Protoglobin (Pgb) is a recently discovered haem-protein with distinct structural and functional features that make it unique within the globin superfamily. The MaPgb* structure can be considered as an expanded version of the 3/3 helical sandwich typical of “classical” globins (i.e. Mb), with an additional N-terminal extension, built by a 20-residue loop, followed by the Z-helix, which precedes the globin-fold conserved A-helix. Residues belonging to the Z-helix contribute to formation of the Pgb homodimer, which is centered on the intermolecular four-helix bundle built by the G- and H-helices of the two subunits. Thus, in Pgb the access of diatomic ligands, such as O2, CO, and NO, to the haem is granted by two orthogonal apolar tunnels that reach the haem distal region from entry sites at the B/G and B/E helix interfaces.

High-resolution data (1.60 Å) on the MaPgb*(III)-cyanide crystals were collected at the ESRF synchrotron facility (ESRF, Grenoble, France), and the structure was refined to a final R-factor and R-free of 17.5% and 23.8%, respectively. In the MaPgb*(III)-cyanide complex the cyanide molecule is bound to the sixth coordination site of the haem-Fe(III) atom, with a coordination bond of 2.16 Å and a Fe-C-N angle of 171° for chain A, and of 2.14 Å and 169° for chain B. Two H-bonds stabilize the haem-Fe(III)-bound cyanide molecule. On one hand, the cyanide N atom is linked to Tyr(61)B10 OH group (2.84 Å and 2.71 Å, for chain A and B, respectively), on the other, it is hydrogen bonded to Trp(60)B9 Nε2 atom (2.98 Å or 2.99 Å). The presence of the haem-Fe(III)-bound cyanide molecule induces a rotation of the Phe(93)E11 side chain around the Cβ-Cγ bond of about 120° relative to the ligand-free MaPgb*(III). The rotation of the Phe(93)E11 side chain allows the rotation of the Trp(60)B9 side chain of ∼90° towards the center of the haem distal site. As a consequence, in the MaPgb*(III)-cyanide complex: (i) tunnel 1 is hindered by the Trp(60)B9 side chain, and (ii) the Trp(60)B9 Nε1 atom is at H-bond distance to the haem-Fe(III)-bound cyanide ligand. Interestingly, the 149–154 region, which faces Trp(60)B9 side chain on one side and the second subunit of the dimer on the other, is significantly divergent in its Cα-backbone relative to the ligand-free MaPgb*(III) and MaPgb*(II)-O2 structures (maximum displacement at Ala(151)G13 of 1.75 Å and 1.64 Å, respectively), and shows signs of structural heterogeneity, with Ile(149)G11 and Thr(152)G14 adopting two alternate conformations. Thus, ligand binding, and the consequent relocation of the Trp(60)B9 side chain within the haem distal cavity, appears to release structural constraints at the dimeric interface. Cyanide binding causes also a shift of about 1 Å of the Tyr(61)B10 backbone toward the interior of the haem distal site, with the concomitant side chain rotation of ∼90° around the Cβ-Cγ bond.

>[2x]MSVEKIPGYTYGETENRAPFNLEDLKLLKEAVMFTAEDEEYIQKAGEVLEDQVEEILDTWYGFVGSHPHLLYYFTSPDGTPNEKYLAAVRKRFSRWILDTSNRSYDQAWLDYQYEIGLRHHRTKKNQTDNVESVPNIGYRYLVAFIYPITATMKPFLARKGHTPEEVEKMYQAWFKATTLQVALWSYPYVKYGDF N-{5-[2-amino-7-(1-hydroxy-2-methylpropan-2-yl)-7H-pyrrolo[2,3-d]pyrimidine-5-carbonyl]pyridin-3-yl}-2-(5-chloropyridin-2-yl)acetamide | C23 H22 Cl N7 O3 | 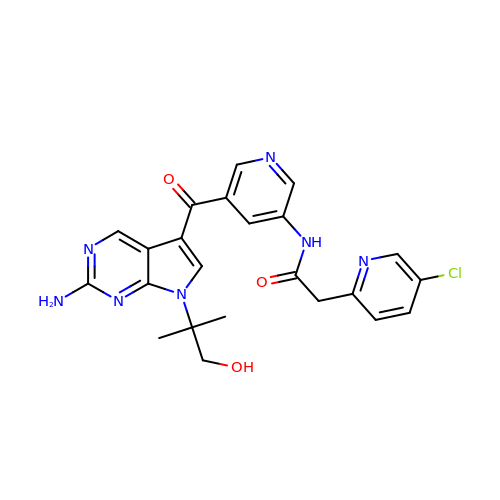BPIWZDNVMQQBQX-UHFFFAOYSA-N>MGHHHHHHGLSSSPSEILQELGKGSTHPQPGVSPPAAPAAPGPKDGPGETDAFGNSEGKELVASGENKIKQGLLPSLEDLLFYTIAEGQEKIPVHKFITALKSTGLRTSDPRLKECMDMLRLTLQTTSDGVMLDKDLFKKCVQSNIVLLTQAFRRKFVIPDFMSFTSHIDELYESAKKQSGGKVADYIPQLAKFSPDLWGVSVCTVDGQRHSTGDTKVPFCLQSCVKPLKYAIAVNDLGTEYVHRYVGKEPSGLRFNKLFLNEDDKPHNPMVNAGAIVVTSLIKQGVNNAEKFDYVMQFLNKMAGNEYVGFSNATFQSERESGDRNFAIGYYLKEKKCFPEGTDMVGILDFYFQLCSIEVTCESASVMAATLANGGFCPITGERVLSPEAVRNTLSLMHSCGMYDFSGQFAFHVGLPAKSGVAGGILLVVPNVMGMMCWSPPLDKMGNSVKGIHFCHDLVSLCNFHNYDNLRHFAKKLDPRREGGDQRHSFGPL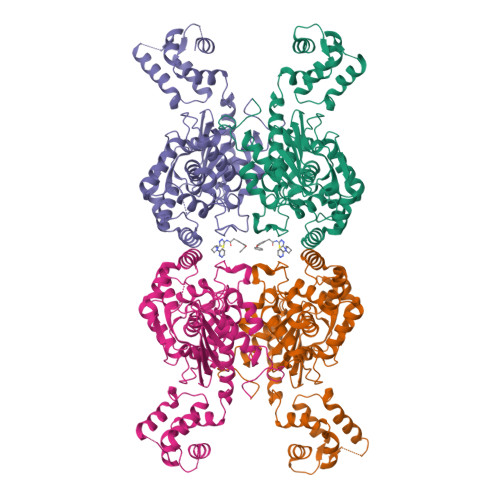DYESLQQELALKETVWKKVSPESNEDISTTVVYRMESLG[4x]> GPLGSMQRINNAIDSLIGHLVPAAAGDDDDARTRRQAVFDLVRALLEQPGSNIPSDVNHASDLIKRRLISTNPSQALRFSNLYTRL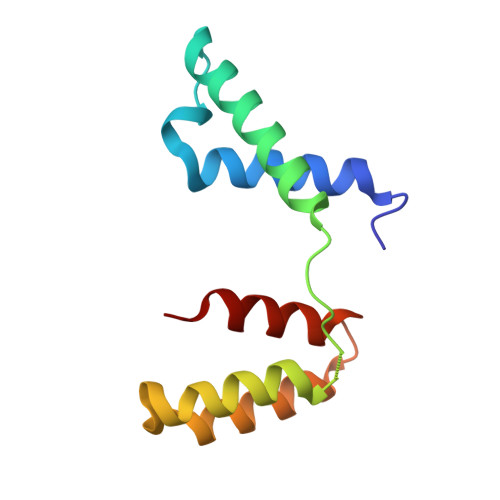LALPVLNQKWAILYLLHQLAD> AG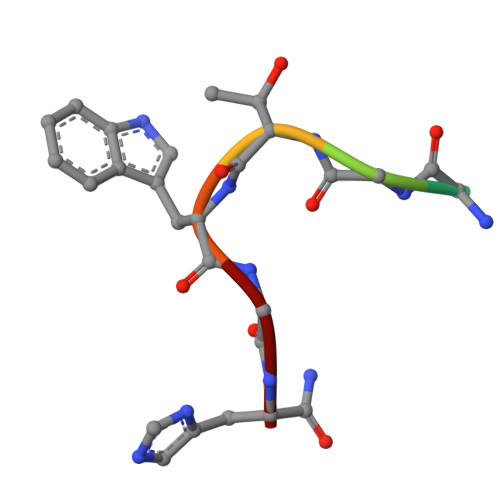HTWGH5-ethyl-2-{[2-methoxy-4-(4-methylpiperazin-1-yl)phenyl]amino}-11-methyl-5,11-dihydro-6H-pyrimido[4,5-b][1,4]benzodiazepin-6-one | C26 H31 N7 O2 | 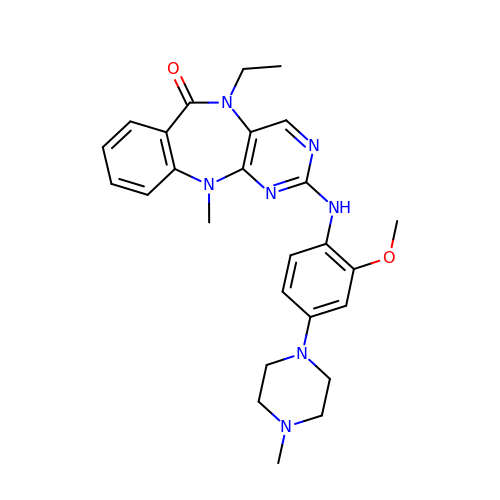REPCEIPSIPNRSG-UHFFFAOYSA-N> MDTSTTASVASANASTSTSMAYDLGSMSKDDVIDLFNKLGVFQAAILMFAYMYQAQSDLSIAKFADMNEASKESTTAQKMANLVDAKIADVQSSSDKNAKAQLPDEVISYINDPRNDITISGIDNINAQLGAGDLQTVKAAISAKANNLTTTVNNS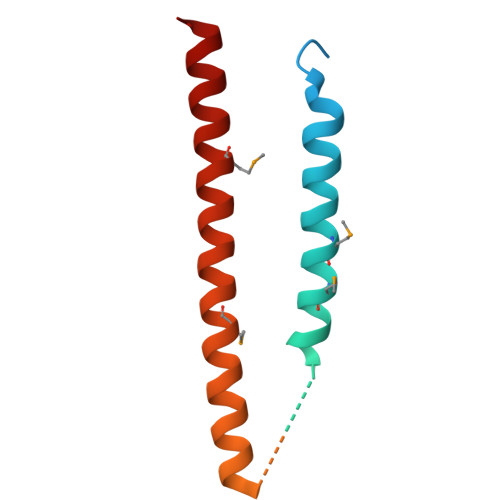QLEIQQMSNTLNLLTSARSDMQSLQYRTISGISLGK>GSMADEALF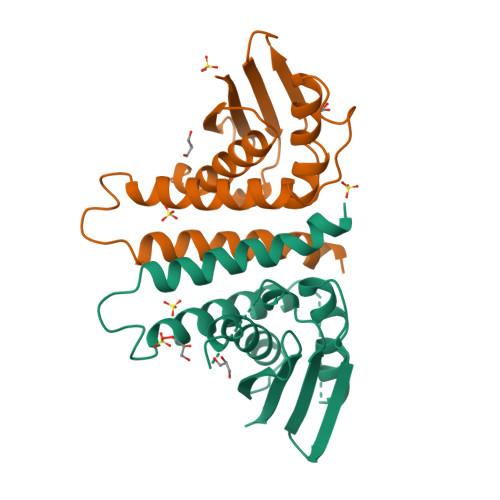LLLHNEMVSGVYKSAEQGEVENGRCITKLENMGFRVGQGLIERFTKDTARFKDELDIMKFICKDFWTTVFKKQIDNLRTNHQGIYVLQDNKFRLLTQMSAGKQYLEHASKYLAFTCGLIRGGLSNLGIKSIVTAEVSSMPACKFQVMIQKL[2x]2,4-di~{tert}-butylphenol | C14 H22 O | 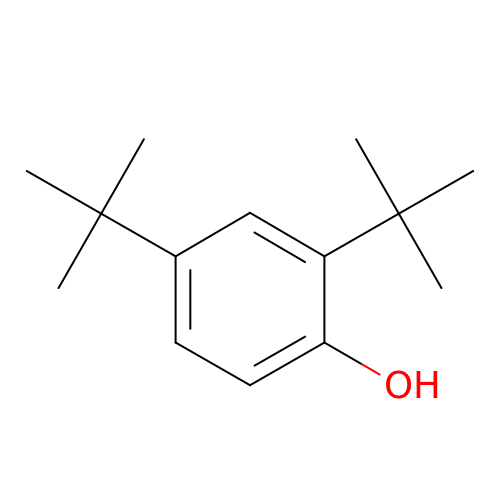ICKWICRCANNIBI-UHFFFAOYSA-N> TDL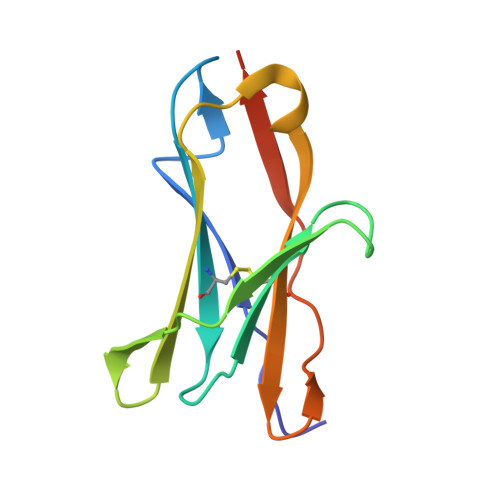PRPSISAEPGTVIPLGSHVTFVCRGPVGVQTFRLERERNYLYSDTEDVSQTSPSESEARFRIDSVNAGNAGLFRCIYYKSRKWSEQSDYLELVVKGEDVTWA> MQNITQSWFVQGMIKATTDA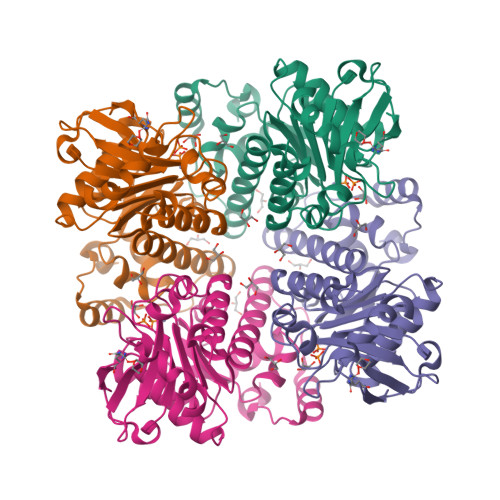WLKGWDERNGGNLTLRLDDADIAPYHDNFHQQPRYIPLSQPMPLLANTPFIVTGSGKFFRNVQLDPAANLGIVKVDSDGAGYHILWGLTNEAVPTSELPAHFLSHCERIKATNGKDRVIMHCHATNLIALTYVLENDTAVFTRQLWEGSTECLVVFPDGVGILPWMVPGTDAIGQATAQEMQKHSLVLWPFHGVFGSGPTLDETFGLIDTAEKSAQVLVKVYSMGGMKQTISREELIALGKRFGVTPLASALAL>MAHHHHHHMQTQTQTQPAGNAFQYEIRDISLAEFGRKEINLAEHEMPGLMQTREKYGAEQPLKGVRLAGSLHMTIQTAVLIETLQALGANVRWCSCNIFSTQDHAAAAIVAAGTPVFAWKGETLEEYWECTWKTLLFPDDMGPQLIVDDGGDATLMVHRGFYAEDNPSILDDDEGSEELAIVNKLLKRIQKEKPGYWHKIVPELKGVSEETTTGVHRLYEMMKEGKLLFPALNVNDSVTKSKFDNVYGCRHSLVDAIMRA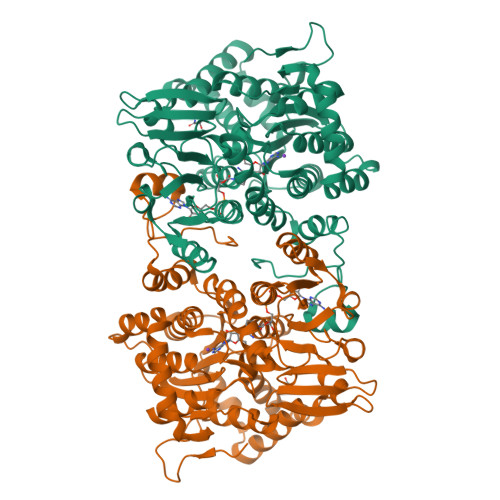TDVMLSGKVACVLGYGDVGKGSAESLKGQGARVVVTEVDPICALQACMAGYEVVRIEDVLDKAEIFVTTTGNCDIIRIEHMEKMRHNAIVCNIGHFDNEIQVKALKEFPGIKRIEIKPQVDQFVFPDGHAIVLLAEGRLVNLGCATGHPSFVMSNSFTNQTLAQISLWKEKYELGVYTLPKKLDEEVARLHLEKLGAKLTVLTDKQAKYLGIAKDGPYKPDHYRY[4x]> MNGVYDVGGTDGLGPINRPADEPVFRAEWEKVAFAMFPATFRAGFMGLDEFRFGI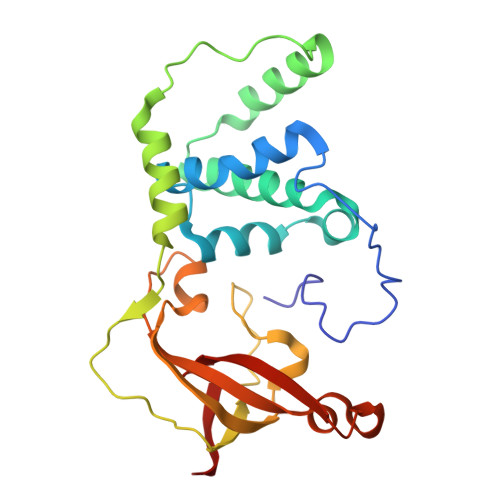EQMNPAEYLESPYYWHWIRTYIHHGVRTGKIDLEELERRTQYYRENPDAPLPEHEQKPELIEFVNQAVYGGLPASREVDRPPKFKEGDVVRFSTASPKGHAKRARYVRGKTGTVVKHHGAYIYPDTAGNGLGECPEHLYTVRFTAQELWGPEGDPNSSVYYDCWEPYIELVDT methyl 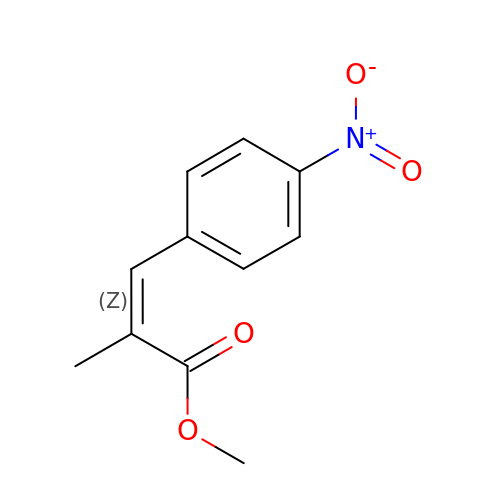(~{Z})-2-methyl-3-(4-nitrophenyl)prop-2-enoate | C11 H11 N O4 | PSKQMOVEPBBTCO-FPLPWBNLSA-N>[4x]MREKGRRQAVRGPAFMFNDRGTSLTAEEERFLDAAEYGNIPVVRKMLEESKTLNVNCVDYMGQNALQLAVGNEHLEVTELLLKKENLARIGDALLLAISKGYVRIVEAILNHPGFAASKRLTLSPCEQELQDDDFYAYDEDGTRFSPDITPIILAAHCQKYEVVHMLLMKGARIERPHDYFCKCGDCMEKQRHDSFSHSRSRINAYKGLASPAYLSLSSEDPVLTALELSNELAKLANIEKEFKNDYRKLSMQCKDFVVGVLDLCRDSEEVEAILNGDLESAEPLEVHRHKASLSRVKLAIKYEVKKFVAHPNCQQQLLTIWYENLSGLREQTIAIKCLVVLVVALGLPFLAIGYWIAPCSRLGKILRSPFMKFVAHAASFIIFLGLLVFNASDRFEGITTLPNITVTDYPKQIFRVKTTQFTWTEMLIMVWVLGMMWSECKELWLEGPREYILQL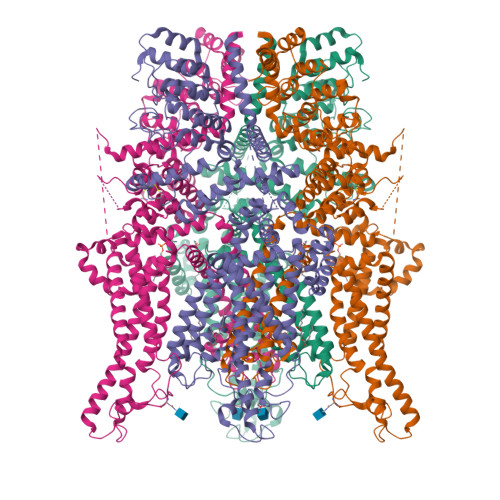WNVLDFGMLSIFIAAFTARFLAFLQATKAQQYVDSYVQESDLSEVTLPPEIQYFTYARDKWLPSDPQIISEGLYAIAVVLSFSRIAYILPANESFGPLQISLGRTVKDIFKFMVLFIMVFFAFMIGMFILYSYYLGAKVNAAFTTVEESFKTLFWSIFGLSEVTSVVLKYDHKFIENIGYVLYGIYNVTMVVVLLNMLIAMINSSYQEIEDDSDVEWKFARSKLWLSYFDDGKTLPPPFSLVPSPKSFVYFIMRIVNFPKCRRRRLQKDIEMGMGNSKSRLNLFTQSNSRVFESHSFNSILNQPTRYQQIMKRLIKRYVLKAQVDKENDEVNEGELKEIKQDISSLRYEL> AVPIAQKSEPHSLSSEALMRRAVSLVTDSTSTFLSQTTYALIEAITEYTKAVYTLTSLYRQYTSLLGKMNSEEEDEVWQVIIGARAEMTSKHQEYLKLETTWMTAVGLSEMAAEAAYQTGADQASI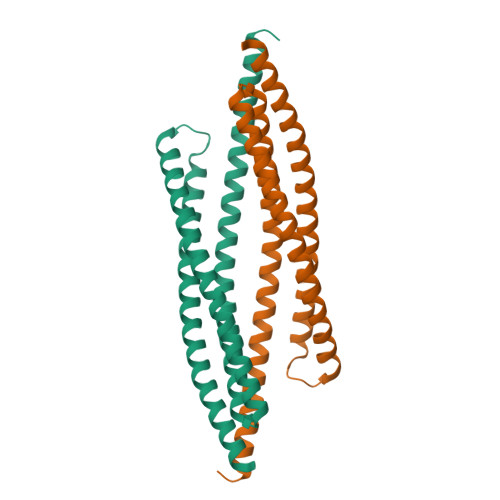TARNHIQLVKLQVEEVHQLSRKAETKLAEAQIEELKQKTQEEGEERAESEQEAYLRED>[2x]GPAGKATANAPTDAAITAASDFAALEKACAGRLGVTLLDTASGRRIGHRQDERFPMCSTFKSMLAATVLSQAERMPALLDRRVPVGEADLLSHAPVTRRHAGKDMTVRDLCRATIITSDNTAANLLFGVVGGPPAVTAFLRASGDTVSRSDRLEPELNSFAKGDPRDTTTPAAMAATLQRVVLGEVLQPASRQQLADWLIDNETGDACLRAGLGKRWRVGDKTGSNGEDARNDIAVLWPVAGGAPWVLTAYLQAGAISYEQRASVLAQVGRIADRLIG

Of particular clinical importance is the widely disseminated class A SBLs, including the mobile, plasmid-encoded extended-spectrum CTX-M and carbapenem-hydrolyzing KPC families (both produced in opportunistic Gram-negative bacteria, such as Klebsiella pneumoniae, Pseudomonas aeruginosa, and Escherichia coli), as well as chromosomally encoded L2 from Stenotrophomonas maltophilia (a lung colonist of cystic fibrosis patients). SBLs hydrolyze antibiotics via formation of a hydrolytically labile acyl enzyme intermediate, while MBL catalysis proceeds without a covalent intermediate. The diazabicyclooctanes (DBOs), including avibactam, relebactam, and others, are a new BLI class with improved activity against a wider range of SBL targets than classic BLI scaffolds. DBOs inhibit SBLs through covalent formation of a carbamyl ester to the active-site serine concomitant with DBO ring opening.

L2 (an SBL) is one of two intrinsic β-lactamases, with L1 (an MBL), which together provide resistance to all β-lactams, making S. maltophilia one of the most extensively drug-resistant pathogens in the clinic and one of the most difficult to treat. For L2 (Kiapp, 2.7 μM), both the second-order carbamylation rate constant (4,000 ± 620 M−1 s−1) and off-rate (0.00055 ± 0.00021 s−1) are relatively high. Relebactam cocomplex structures were obtained after 16-h soaks for CTX-M-15 (1.12 Å, P212121), L2 (1.78 Å, P212121), KPC-2 (1.04 Å, P21212), KPC-3 (1.06 Å, P21212), and KPC-4 (1.04 Å, P21212). For L2, electron density consistent with a single conformation of relebactam (refined at full occupancy) was observed in one of the two molecules in the asymmetric unit (chain B). Consistent with previous observations for other potent L2 inhibitors in this crystal form, we observe a noncovalently bound molecule from the crystallization solution (d-serine) in the chain A active site. In addition, the L2 structure contains two active-site water molecules uniquely observed bridging relebactam and residues Tyr272, Arg244, Lys234, and Gly236. In L2, two conformations of His105 are observed on relebactam binding, with one configuration the same as that observed in the L2:avibactam and native structures, which each contain a single His105 conformation. As in CTX-M-15, these movements are not observed in unliganded enzyme or in the avibactam-bound L2 structure. These energetically unfavorable clashes may indicate why relebactam is 30-fold worse than avibactam at inhibiting L2. In the complex with L2, which contains intact (i.e., nondesulfated but ring-opened) relebactam in a single conformation, Lys73 and Ser130 were similarly close to one another. Despite this proximity, Ser130 is ∼3.9 Å away from the N6 nitrogen, and so relebactam appears to still not be primed for recyclization in L2.> EEQWAREIGAQLR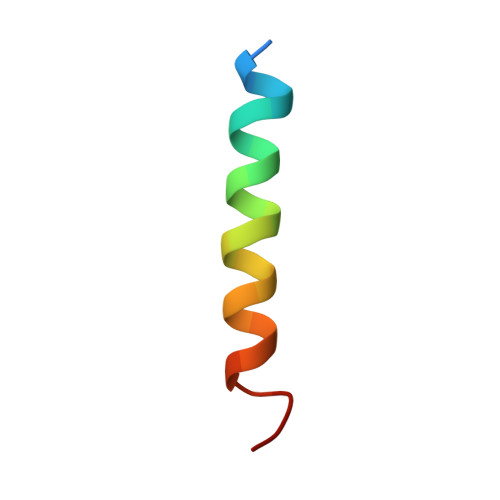RMADDLNAQYERR2-[(R)-{[4-(3-methoxypropoxy)-3-methylpyridin-2-yl]methyl}sulfinyl]-1H-benzimidazole 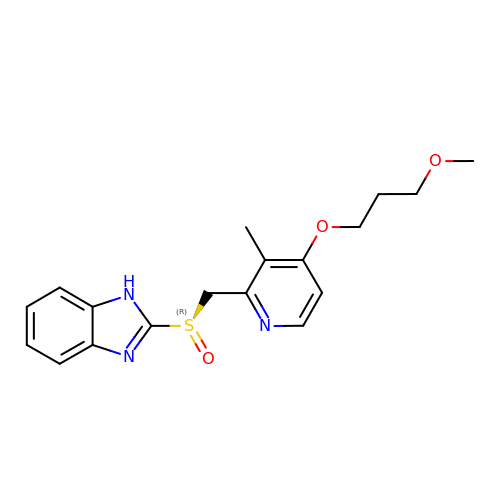| C18 H21 N3 O3 S | YREYEVIYCVEVJK-RUZDIDTESA-N>[6x]MSGSHHHHHHSGSMSERPSDLVVNRLVLFVVKGTATSTHNTVKPLILLEELGVPHDIYVVEKVSAPWFSEINPHKMVPAILDRSPDGRDTLRAWESTSTLMYIADAYDKDGTFGGRNVQERSEINNWLTLHTAALGPTAGYWLYFYK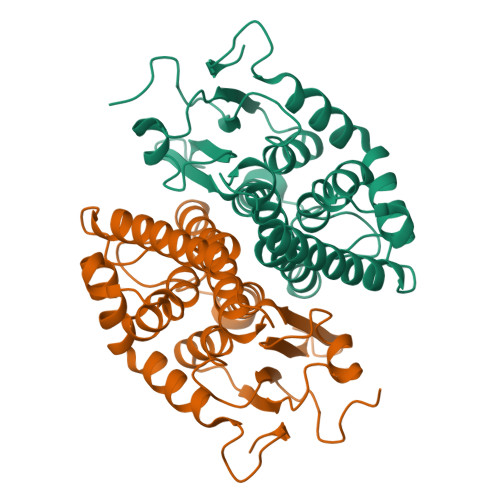LHPEKLPKTIEKLRSNITVQYDILERRLNEPGQQYLALKDRPTIADIATLPFAMKSTAELFGLEFEKWPKLQEWSVRMGEREAVKRAWQRVAGFGHGEKEYGMLEA> GPDSMALFHVDVEGDEIL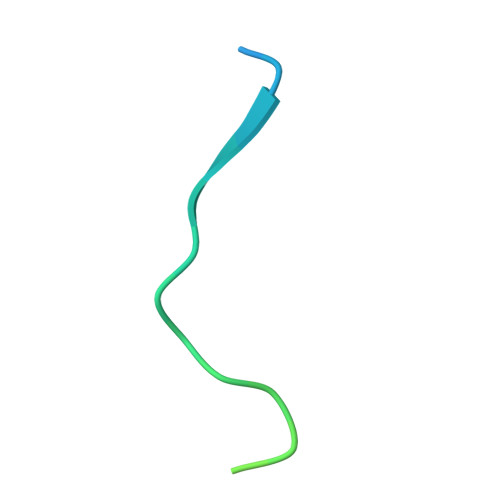KNKLIKRKQIKKVLKSKEIL> VGSLNCIVAVSQNMGIGKNGDLPWPPLRNEGRYFQRMTTTSSVEGKQNLVIMGKKTWFSIPEKNRPLKGRINLVLSRELKEPPQGAHFLSRSLDDALKLTEQPELANKVDMVWIVGGSSVYKEAMNHPGHLKLFVTRIMQDFESDTFFPEIDLE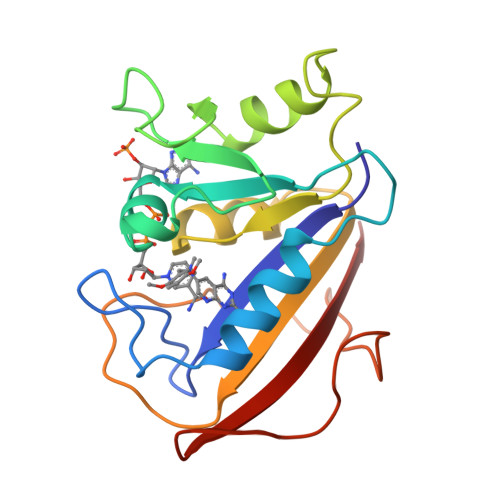KYKLLPEYPGVLSDVQEEKGIKYKFEVYEKND>GSHMSRVQLALRVPDLEASIGFYSKLFGTGPAKVRPGYANFAIAEPPLKLV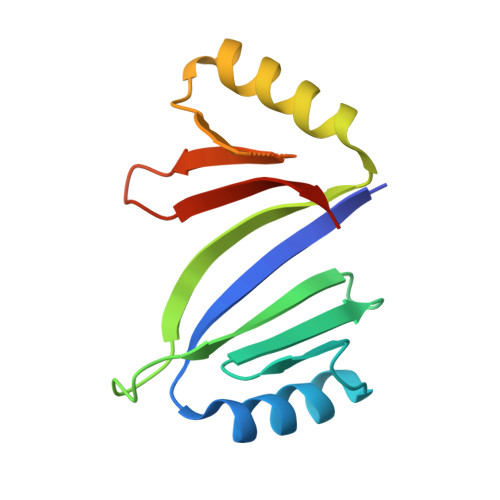LIEGAGEDATRLDHLGVEVEDSAQVGHAARRLKESGLATVEENDTACCHAFQDKVWVTGPGGEPWEVYVVKGDAD[4x]>[4x]M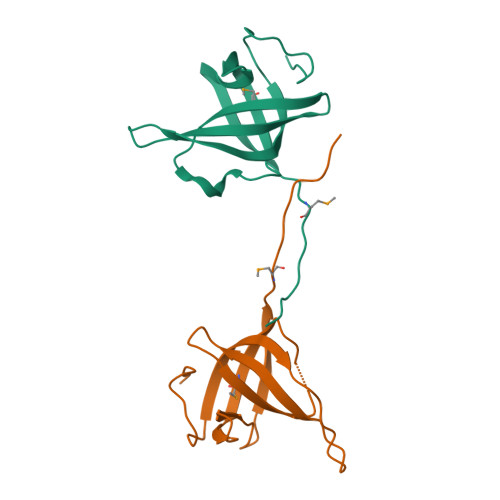TTETFVKDIKPGLKNLNLIFIVLETGRVTKTKDGHEVRTCKVADKTGSINISVWDDVGNLIQPGDIIRMTKGYASVFKGCLTLYTGRGGDLQKIGEFCMVYSEVPNFSHHHHHH> FSGSEATAAILSRAPWSLQSVNPGLKTNSSKEPKFTKCRSPERETFSCHWTDEVHHGTKNLGPIQLFYTRRNTQEWTQEWKECPDYVSAGENSCYFNSSFTSIWIPYCIKLTSNGGTV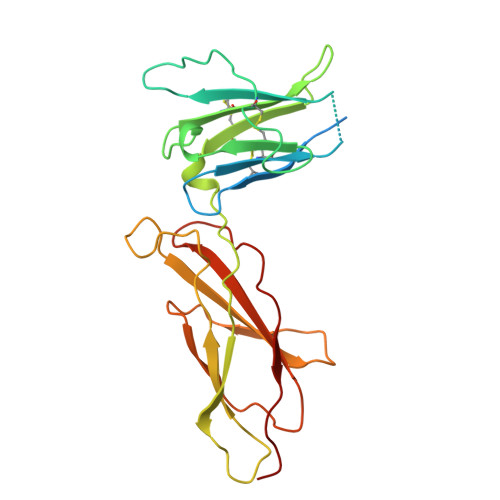DEKCFSVDEIVQPDPPIALNWTLLNVSLTGIHADIQVRWEAPRNADIQKGWMVLEYELQYKEVNETKWKMMDPILTTSVPVYSLKVDKEYEVRVRSKQRNSGNYGEFSEVLYVTLPQMS Short prokaryotic Argonaute proteins (Agos) are associated with NADase domain-containing proteins (TIR-APAZ or SIR2-APAZ) encoded in the same operon. They confer immunity against mobile genetic elements, such as bacteriophages and plasmids, by inducing NAD+ depletion upon recognition of target nucleic acids. Target DNA binding triggers tetramerization of the TIR-APAZ/Ago complex by a cooperative self-assembly mechanism, while the heterodimeric SIR2-APAZ/Ago complex does not assemble into higher-order oligomers upon target DNA binding. However, the NADase activities of these two systems are unleashed via a similar closed-to-open transition of the catalytic pocket, albeit by different mechanisms.

To investigate the interaction mode between TIR-APAZ and Ago proteins, we first co-purified the binary complex from Maribacter polysiphoniae (termed TIR-APAZ/Ago complex hereinafter, also known as SPARTA)30 and determined its cryo-EM structure in the presence of gRNA. We were able to build the structure of most regions of the TIR-APAZ/Ago complex, with the exception of the C-terminal region (aa 419–452) of TIR-APAZ and residues 161–200 of the Ago protein. Although the majority of the gRNA could not be resolved, two nucleotides (2G–3A), defined as the seed region, could be clearly seen. This observed seed region is much shorter in length than the seed sequences pre-organized by other previously reported eAgos and pAgos. In the TIR-APAZ/Ago–gRNA ribonucleoprotein (RNP) complex structure, the Ago protein is bracketed by the separated TIR and APAZ domains of TIR-APAZ protein, which are connected by a helix (aa 146–158) and the following loop, termed here as the bridging region. Ago protein, together with the APAZ domain of APAZ-TIR protein, creates a positively charged channel to potentially accommodate the gRNA–target DNA heteroduplex. The RNP complex structure is nearly identical to the apo TIR-APAZ/Ago structure predicted by AlphaFold36, with an RMSD of 0.936 Å, suggesting that gRNA has little impact on the configuration of TIR-APAZ/Ago complex, possibly due to the short pre-organized seed sequence or the lack of PAZ domain, which is absent in short pAgo system. The TIR domains in both apo TIR-APAZ/Ago and RNP complexes are catalytically inactive, but target ssDNA binding could efficiently activate the NADase activity. Therefore, our structures presumably explain why target ssDNA binding initiates the dimerization of Ago proteins. It is intriguing to note that a long loop (aa 314–332) protruding from the PIWI domain in the target-free complex would pose steric barriers to the propagation of the gRNA–DNA duplex at ~13–15 bp positions. In the resting state, the NADase activity of TIR is likely to be self-inhibited partially by the flexible BB-loop.

> MKELIYIEEPKILFAHGQKCTDARDGLALFGPLNNLYGIKSGVIGTKQGLKIFRDYLDHIQKPIYNSNSITRPMFPGFEAVFDCKWESTGITFKEVTNEDIGKFLYNSSTHKRTYDLVSLFIDKIISANKNEDENVDVWFVIVPDEIYKYCRPNSVLPKEMVQTKALMSKSKAKSFRYEPSLFPDINIELKEQEKEAETYNYDAQFHDQFKARLLKHTIPTQIFRESTLAWRDFKNAFGLPIRDFSKIEGHLAWTISTAAFYKAGGKPWKLSDVRNGVCYLGLVYKKVEKSKNPRNACCAAQMFLDNGDGTVFKGEVGPWYNPKNGQYHLEPKEAKALLSQSLQSYKEQIGEYPKEVFIHAKTRFNHQEWDAFLEVTPKETNLVGVTISKTKPLKLYKTEGDYTILRGNAYVVNERSAFLWTVGYVPKIQTALSMEVPNPLFIEINKGEADIKQVLKDILSLTKLNYNACIFADGEPVTLRFADKIGEILTASTDIKTPPLAFKYYI;> MRNKIFISHATPDDNDFTRWLALKLIGLGYEVWCDILFLDKGVDFWSNIEKVIREDTCKFLLVSSSYSNQREGVLKELAVAAKVKKQLKDDKFIIPLAIDEQLSYDDINIDIVRLNAIDFKMSWARGLKDILEAFEKQKVPKEVADASKSNLLYQQIFLHDKSVIEKEEIYDSNWLSILSFPEELRFHEYNWMLPKRFDVRELTFPAVRYKNYLCTFAWAYDFTYHLPKTETYHKSKTIRIPTEEILSGSYDSNFIRNAECKRLIVQLLNKAFELRMKDKEVQEYEMSNKTAYWLEKGKLEKDKFEKTMLVGKQKDKNWHFAISGASKLYPFPVLMISSHIFFTADGKKLIDSSSVQHSSRRRQGKNWWNNTWRTKLLAFIKYLSDDDTSFYLEMGSEEKVFVSNEPVKFKGNVSYNIPEKNTLEEEAELSGFNQGEDIEELEELIENLEAE>[4x]SPLAAYEVDDSTGYLTSDVGGPIQDQTSLKAGIRGPTLLEDFMFRQKIQHFDHERVPERAVHARGAGAHGTFTSYADWSNITAASFLNATGKQTPVFVRFSTVAGSRGSADTARDVHGFAT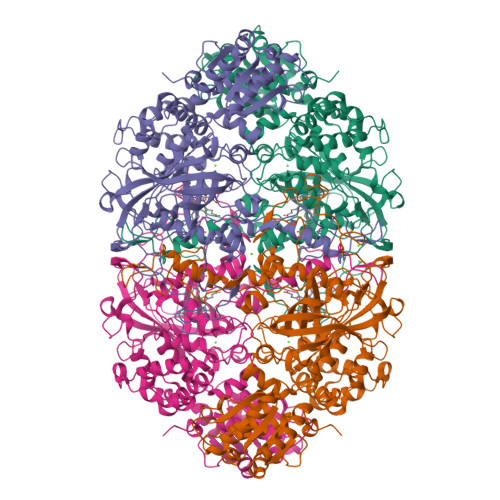RFYTDEGNFDIVGNNIPVFFIQDAIQFPDLIHSVKPRPDNEIPQAAFAHDSAWDFFSQQPSTMHTLFWAMSGHGIPRSYRHMDGFGVHTFRFVKDDGSSKLIKWHFKSRQGKASLVWEEAQVLSGKNADFHRQDLWDAIESGNGPEWDVCVQIVDESQAQAFGFDLLDPTKIIPEEYAPLTKLGLLKLDRNPTNYFAETEQVMFQPGHIVRGIDFTEDPLLQGRLFSYLDTQLNRNGGPNFEQLPINMPRVPIHNNNRDGAGQMFIHRNKYPYTPNTLNSGYPRQANQNAGRGFFTAPGRTASGALVREVSPTFNDHWSQPRLFFNSLTPVEQQFLVNAMRFEISLVKSEEVKKNVLTQLNRVSHDVAVRVAAAIGLGAPDADDTYYHNNKTAGVSIVGSGPLPTIKTLRVGILATTSESSALDQAAQLRTRLEKDGLVVTVVAETLREGVDQTYSTADATGFDGVVVVDGAAALFASTASSPLFPTGRPLQIFVDAYRWGKPVGVCGGKSSEVLDAADVPEDGDGVYSEESVDMFVEEFEKGLATFRFTDRFALDS>GSKTIRKLLSFTSNDILRFDKAYDENDVQEFVNLCSSTCEIEKLEDRMHPWAADPKTIGALSATQLAILASKENEPHYKDAIREANGIAVFINLLKSHELDRVHAAVVALSFLSVDNVKNCICMFESGALPYLISGMKSNIDGMKAACAQTCRNIFVLDKKYKKEFLKLGGITQLVNLLELPSNYDDSQPLYTQLEAIYHLEDFILNDGDEIPEFLEAVKNSNSIKNLKTLQQCPEQD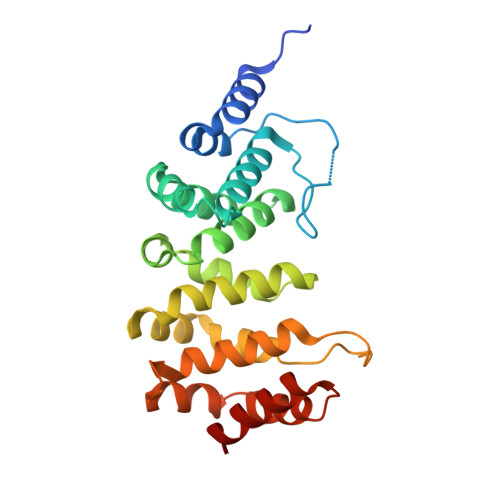LAEASNVLLLRLTD[2x]> VPATRILLLVLA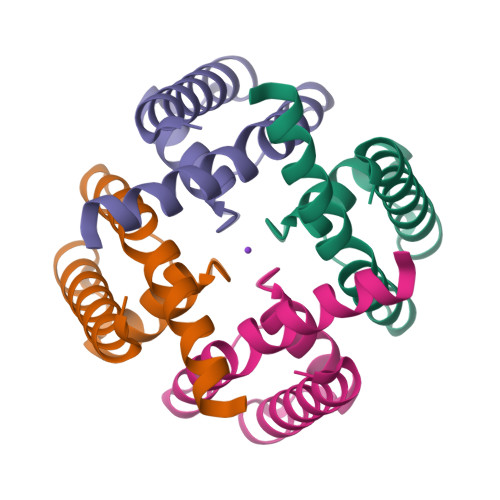VIIYGTAGFHFIEGESWTVSLYWTFVTIATVGYGDYSPHTPLGMYFTCTLIVLGIGTFAVAVQRLLEFLI The abnormal expansion of GGGGCC (G4C2) repeats in the noncoding region of the C9orf72 gene is a major genetic cause of two devastating neurodegenerative disorders, amyotrophic lateral sclerosis (ALS) and frontotemporal dementia (FTD). These G4C2 repeats are known to form G-quadruplex (G4) structures, which are hypothesized to contribute to disease pathogenesis. In the present study, we isolated and characterized two distinct G4 topologies formed by four-repeat G4C2 DNA (d(G4C2)4): a dimeric parallel form (d(G4C2)4-para) and a monomeric antiparallel form (designated d(G4C2)4-anti). The fundamental structural unit of G4s, known as the G-tetrad, is composed of four guanine bases arranged in a square planar structure via cyclic Hoogsteen hydrogen bonding.

The asymmetric unit contains four independent oligonucleotide chains, designated chains A through D, with well-resolved electron density for most nucleotides, except for the 3′-flanking bases C23, C24, and loop residues C11 and C12. The crystal structure reveals a monomeric antiparallel chair-type G4 composed of four stacked G-tetrads in which the hydrogen-bond directionalities are clockwise (G1→G10→G13→G22), anti-clockwise (G2←G9←G14←G21), clockwise (G3→G8→G15→G20), and anti-clockwise (G4←G7←G16←G19) patterns with all Hoogsteen hydrogen bonds of N1-O6 and N2-N7 from the electron pair acceptor to the electron pair donor. Three centrally aligned K+ ions stabilize the G-core by coordinating with the guanine O6 atoms of the tetrads and an additional K+ ion is observed between bases C6, C18, and the G4·G7·G16·G19 tetrad layer. The glycosidic conformations of the guanines alternate in a syn·anti·syn·anti pattern, consistent with the antiparallel topology. The G-core is connected by three edgewise CC loops, resulting in two wide grooves with widths of 21.5/21.7 Å and two narrow grooves with widths of 8.5/8.9 Å. The first and third loops containing C5, C6, C17, and C18 (at the bottom) span narrow grooves, while the second loop composed of C11 and C12 (on the top) spans a wide groove. In contrast, the C6 and C18 bases stack onto the G4·G7·G16·G19 G-tetrad layer in coordination with a K+ ion forming an antiprismatic coordination environment with distances of 2.6 Å and 3.0 Å from the O2 atom of C6 and the O2 and N3 atoms of C18. Structural alignment revealed that d(G4C2)4-anti is similar to NAN, with an RMSD of ∼0.722 Å, indicating a conserved architecture composed of four G-tetrad layers and three lateral loops. In contrast, d(G4C2)4-anti had a molecular weight of 6.8 ± 0.5 kDa, which corresponds well with the theoretical monomeric molecular weight (7.5 kDa).

>[4x]GGGGCCGGGGCCGGGGCCGGGGCC>EPYTDSNVPEGDSVPEAHWTKLQHSLDTALAAARSAPTAPIAARVTGQTRNITVDPRLFKAARLHSPRVLFSTQPPPTSSDTLDLDFQAHGTIPFNRTHRSAASSTHPVFHMGEFSVCDSVSVWVGDKTTATDIKGKEVTVLAEVNINNSVFRQYFFETKCRASNPVESGCRGIDSKHWNSYCTTTHTFVKALTTDEKQAAWRFIRIDTACVCVLSRKATAAGHHHHHHH[2x];>[2x]ADPKETCSTGLYTHSGECCKACNLGEGVAQPCGADQTVCEPCLDSVTFSDVVSATEPCKPCTECLGLQSMSAPCVEADDAVC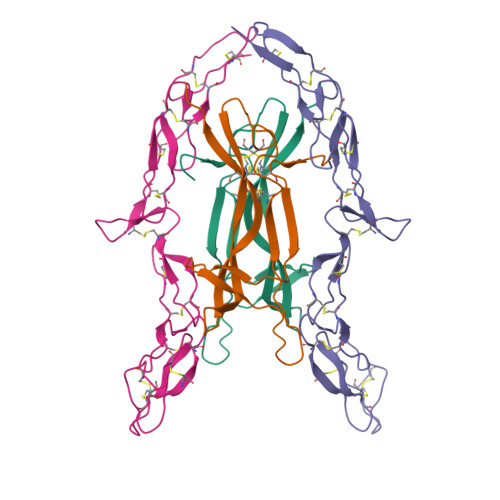RCAYGYYQDEETGHCEACSVCEVGSGLVFSCQDKQNTVCEECPEGTYSDEANHVDPCLPCTVCEDTERQLRECTPWADAECEHHHHHHH> MAHWTRFERDQEGDIKKLVSLMSGIQDDQDGNFQQALQFAWSNFRFHRYLDVSSHTVLRTLEGIFEKLVVHSDLEKAESWKRLTEEFLLLPLPNTEGTKTDSHFAVLSLLLCLSDSPSNHDYTEKPRKKENDEQEPFDWGKYLREGEDIEFSPDADTPEWSEASEEEDAQEPPSREDSGIQVDRTPLEDPEKKGAPPLVSWKVGEPDARSWLEQHIVHQYWTSRAPRFSHSSHLHSNLSAIWDQHLYTTDPLYTPDDKTIVTETQVIRETLWLLSGVKKLLIFQLNDGKVNVRNDIIVTHMTQNCLRSVLEQIAAYGQVVFRLQKFIDEITGHGSEVPLPGTLPTAKKTTEAPFRTYQAFMWALYKYFISFKEELTEIEKCIINKDETVTLAIVLDKLAPRLAQLKVLHRVFSTGIAEVPPDTRNVVRASHLLNTLYKAILDYDNVGEASEQTVSLLFCLWVETVRPYLEIVDEWIVHGNLFDPAKEFIIQRNKDVPFNHRDFWYATYTLYSVSEKTENEDKMSDNASASSGSDQAPAGRQHTMVSFLKPVLKQIIMAGKSMQLLKNLKCRTALQQDSSRDSDRKSLYTLFLESVQSRLQHGNDSVPDIITEQQVNKLSLIKMQSIVAKHLELDEVHDPLLAINFVRLYLEQSDFLETFTCNEVCVDRSSESVTCQSFELTLRSCLYPHIGKQYLECCGNLMYTLKKDYRLVEYLQAMRNFFLLEAGDTMYDFYTPIFDKIREKEPWLNLSYLNVQIQEAVGQRYPDDSTRLSVSFESVDLAKKKLPVHTLDGLILSYKVPWPVDIVISSECQKIYNQVFLLLLLIKWAKYSLDVLQFNELGNASENESTKEGATVEPFPLPPLTSPSEPKG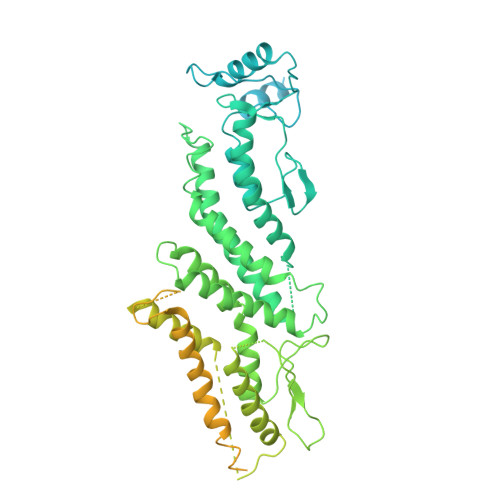QQIHRMFLLRVKLMHFVNSLHNYLMTRILHSTGLEFQHQVEEAKDLDQLIKIHYRYLSTIHDRCLLREKVSSVKEAIMKVLNVVLMFADRWHAGLGAWKKESIVKMESDFTNCHKFLVKVLNKAVCRGSFPHLESLALSLMAGMEQS>[3x]MPKGIALALGLNAVDPKHYGGWAGKLNACEADAEDMAAIAAERGFAVTTLMTKAATRAKVIDAIGKAAKALGKGDIFMLSYSGHGGQVPDTSNDEPDGVDETWCLFDGELIDDELYALLGKFAAGVRVLVFSDSCHSGTVVKMAYYNGTTAARSAGPDEGEIRYRAMPQSVAMRTYRANREFYDTIQQKTKKVDLADVKASILLISGCQDNQLSQDGAFNGAFTGQLLRVWKNGLYKGSYRSFHKAI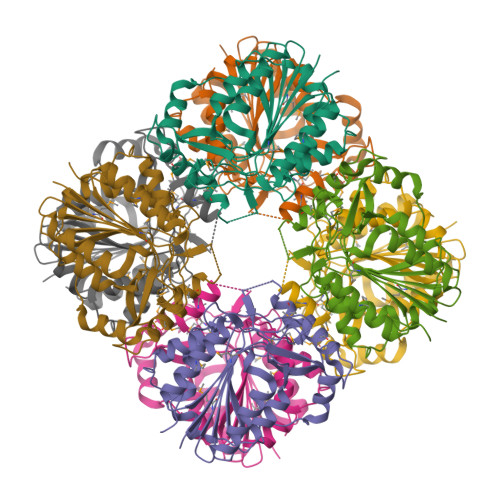VRRMPPDQTPNFFTAGTPDPAFLKQRPFTVLEHHHHHH>[3x]SIGPVADLTISNGAVSPDGFSRQ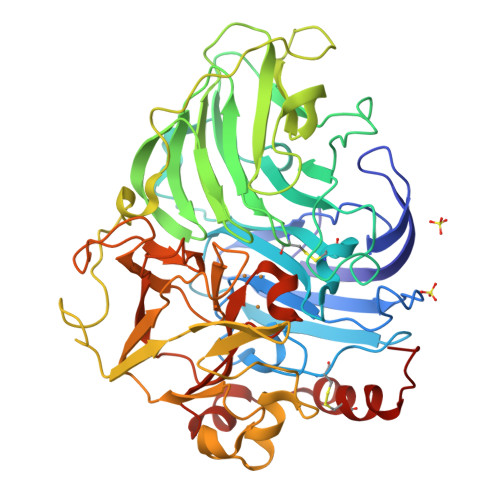AILVNDVFPSPLITGNKGDRFQLNVIDNMTNHTMLKSTSIHWHGFFQHGTNWADGPAFVNQCPISTGHAFLYDFQVPDQAGTFWYHSHLSTQYCDGLRGPIVVYDPQDPHKSLYDVDDDSTVITLADWYHLAAKVGPAVPTADATLINGLGRSIDTLNADLAVITVTKGKRYRFRLVSLSCDPNHTFSIDGHSLTVIEADSVNLKPQTVDSIQIFAAQRYSFVLNADQDVDNYWIRALPNSGTRNFDGGVNSAILRYDGAAPVEPTTTQTPSTQPLVESALTTLEGTAAPGNPTPGGVDLALNMAFGFAGGRFTINGASFTPPTVPVLLQILSGAQSAQDLLPSGSVYSLPANADIEISLPATSAAPGFPHPFHLHGHTFAVVRSAGSSTYNYANPVYRDVVSTGSPGDNVTIRFRTDNPGPWFLHCHIDFHLEAGFAVVMAEDIPEVAATNPVPQAWSDLCPTYDALSPDDQ> GPGSDEAAALRAELRDLELEEARL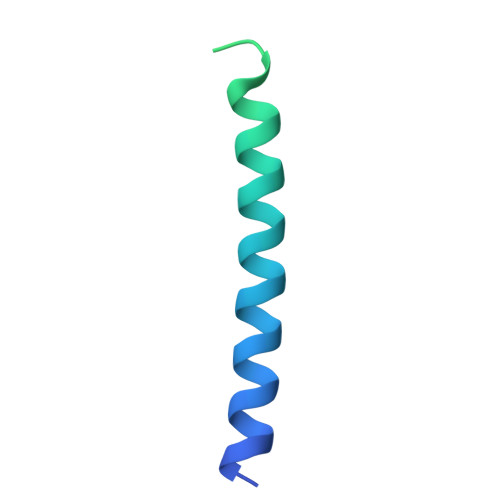VQELEDVDRNNARAAADLQAAQAEAAELDQQERQHYRDYSALKRQQLELLDQLGNVENQLQYARVQLDRLKE> AIGPVADLTLTNAQVSPDGFAREAVVVNGITPAPLITGNKGDRFQLNVIDQLTNHTMLKTSSIHWHGFFQQGTNWADGPAFVNQCPIASGHSFLYDFQVPDQAGTFWYHSHLSTQYCDGLRGPFVVYDPNDPHASLYDIDNDDTVITLADWYHVAAKLGPRFPFGSDSTL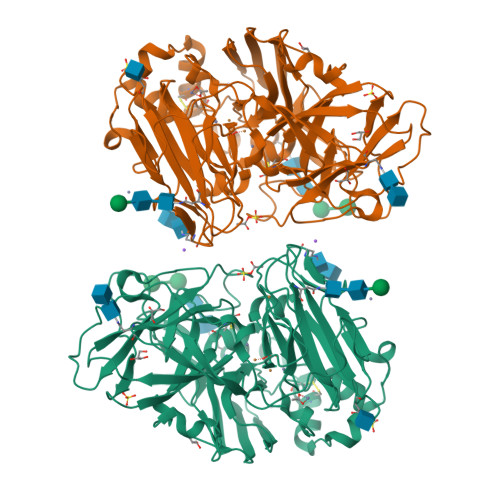INGLGRTTGIAPSDLAVIKVTQGKRYRFRLVSLSCDPNHTFSIDNHTMTIIEADSINTQPLEVDSIQIFAAQRYSFVLDASQPVDNYWIRANPAFGNTGFAGGINSAILRYDGAPEIEPTSVQTTPTKPLNEVDLHPLSPMPVPGSPEPGGVDKPLNLVFNFNGTNFFINDHTFVPPSVPVLLQILSGAQAAQDLVPEGSVFVLPSNSSIEISFPATANAPGFPHPFHLHGHAFAVVRSAGSSVYNYDNPIFRDVVSTGQPGDNVTIRFETNNPGPWFLHCHIDFHLDAGFAVVMAEDTPDTKAANPVPQAWSDLCPIYDALDPSDL>MFENITAAPADPILGLADLFRADERPGKINLGIGVYKDETGKTPVLTSVKKAEQYLLENETTKNYLGIDGIPEFGRCTQELLFGKGSALINDKRARTAQTPGGTGALRVAADFLAKNTSVKRVWVSNPSWPNHKSVFNSAGLEVREYAYYDAENHTLDFDALINSLNEAQAGDVVLFHGCCHNPTGIDPTLEQWQTLAQLSVEKGWLPLFDFAYQGFARGLEEDAEGLRAFAAMHKELIVASSYSKNFGLYNERVGACT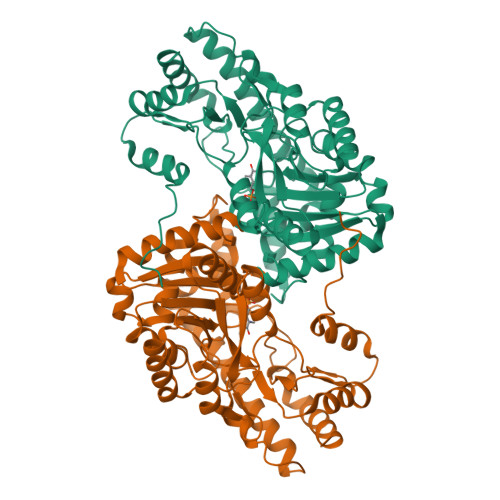LVAADSETVDRAFSQMKAAIRANYSNPPAHGASVVATILSNDALRAIWEQELTDMRQRIQRMRQLFVNTLQEKGANRDFSFIIKQNGMFSFSGLTKEQVLRLREEFGVYAVASGRVNVAGMTPDNMAPLCEAIVAVL[4x]> AEPNRLIKEKSPYLLQHAYNPVDWYPWGEEAFEKARKENKPVFLSIGYSTCHWCHMMAHESFEDEE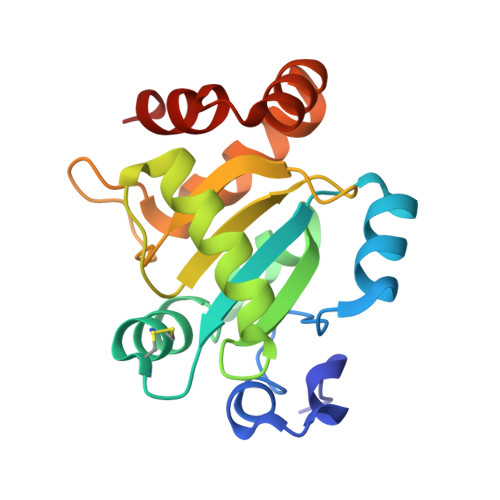VAGLMNEAFVSIKVDREERPDIDNIYMTVCQIILGRGGWPLNIIMTPGKKPFFAGTYIPKNTRFNQIGMLELVPRIKEIWEQQHEEVLDSAEKITSTIQEMIKESSG> MATEPPKIVWNEGKRRFETEDHEAFIEYKMRNNGKVMDLVHTYVPSFKRGLGLASHLCVAAFEHASSHSISIIPSCSY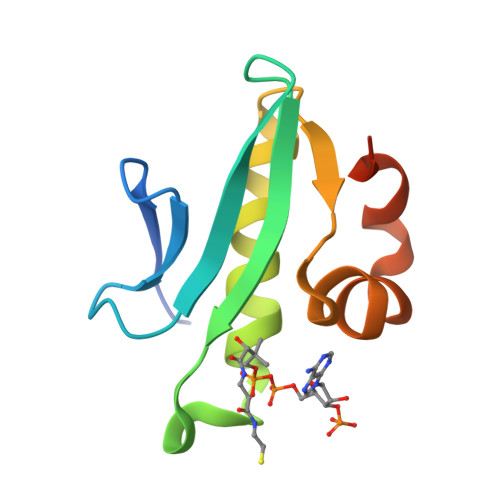VSDTFLPRNPSWKPLIHSEVFKSSI>MQDNSRYTHFLTQHYDAKPQGRDDRYCESIMRRRGLTSPCKDINTFIHGNKRSIKAICENKNGNPHRENLRI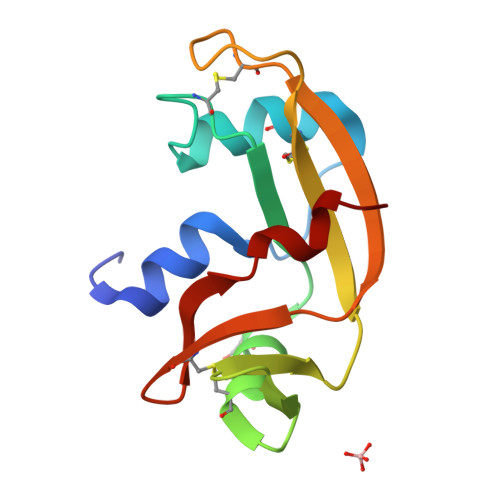SKSSFQVTTCKLHGGSPWPPCQYRATAGFRNVVVACENGLPVRLDQSIFRRP[2x]> GPGSMTERLSLSRDRINVLLLEGISQTAVEYFKSSGYTNVTHLPKALDKADLIKAISSAHIIGIRSRTQLTEEIFAAANRLIAVGCFSVGTNQVELKAARKRGIPVFNAPFSNTRSVAELVIGEIIMLMRRIFPRSVSAHAGGWEKTAIGSREVRGKTLGIVGYGNIGSQVGNLAESLGMTVRYYDTSDKLQYGNVKPAASLDELLKTSDVVSLHVPSSKSTSKLITEAKLRKMKKGAFLINNARGSDVDLEALAKVLQEGHLAGAAIDVFPVEPASNGERFSTPLQGLENVILTPHIGGSTEEAQERIGTEVTRKLVEYSDVGSTVGAVNFPQVQLPPRPTGTRFMHVHENRPGILNSLMNVFSHHHINIASQFLQTDGEVGYLV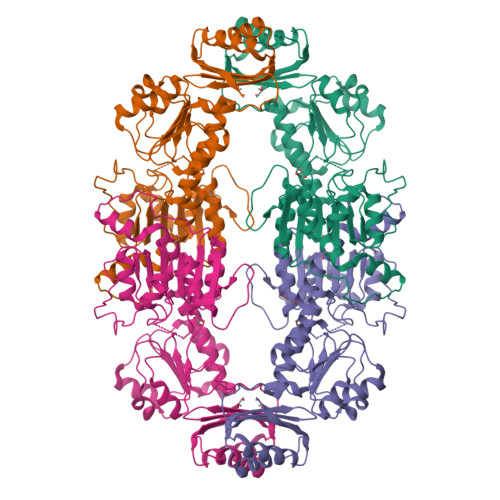MEADGVGEASDAVLQEIREIPGTIRARLLY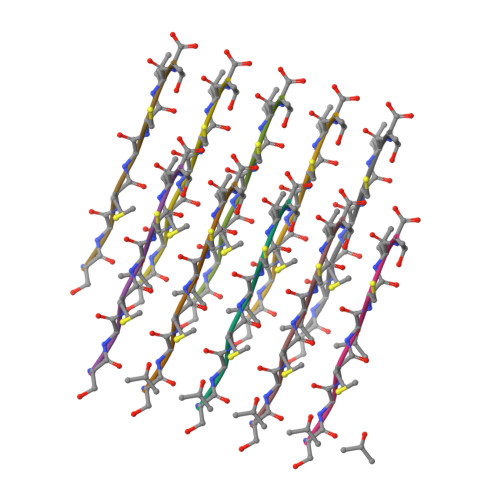> SGMGCIT The TMEM63 family proteins (A, B, and C), calcium-permeable channels in animals that are preferentially activated by hypo-osmolality, have been implicated in various physiological functions. TMEM63s, together with its plant orthologues OSCAs, are members of a newly identified OSCA/TMEM63 cation channel family that are activated by mechanical forces of osmolality. TMEM63 has three members, TMEM63A, B and C in most animals including mouse and human. TMEM63C is essential for maintaining the kidney filtration barrier integrity in zebrafish, and expresses low in chronic kidney disease patients.

Using single-particle cryo-EM, we determined the structure of TMEM63C at 3.56 Å resolution as a monomer. TMEM63C contains 11 transmembrane helices (TMs), TM0-TM10. The N-terminus is oriented towards the extracellular space, while the C-terminus faces the cytosol. Between TM2 and TM3, there is a long cytosolic domain mainly formed by α-helices. Similar to OSCA, the ion-passing pore of TMEM63C is surrounded by TM3-7. The results show that TMEM63C is in closed state with two restriction sites, the radii of which is smaller than 1 Å. Three bulky pore-facing residues (F542, F543 and Y546 on TM6), highly conserved among TMEM63 and OSCA, have been proposed to play critical roles in channel activities. Particularly, the short α-helix located at the cytoplasmic side of TM6 (TM6b) swung to TM4 to avoid the clash with TM0, the intracellular half of which moved close to TM6, compared to that in OSCA. The movement of TM6b may narrow the ion-passing pore of TMEM63C for calcium entrance. Additionally, we identified two non-protein densities within our cryo-EM map of TMEM63C, which are likely composed of lipids, and may contribute to the modulation of mechanosensitive ion channels gating.

> MSAFPDSMDQKFHNMTVNECFQSRSTVLQGQPFGGIPTVLVLNIILWVFVVLLYSFLRKAAWDYGRLALLIHNDSLTSLIYGEQSEKSSPSEVSLEAERRDRGFSSWFFNSLTMRDRDLINKCGDDARIYITFQYHLIIFVLILCIPSLGIILPVNYIGTVLDWNSHFGRTTIVNVSTESKFLWLHSLFAFLYFLINLAFMGHHCLGFVPKKSLHFTRTLMITYVPTEIQDPEIISKHFHEAYPGCVVTRVHFCYDVRNLIDLDDQRRHAMRGRLYYTAKAKKTGKVMIKTHPCSRLCFCKCWTCFKEVDAEQYYSELEEQLTDEFNAELNRVQLKRLDLIFVTFQDARTVRRIYDDYKYIHCGRHPKQSSVTTIVKNYHWRVAHAPHPKDIIWKHLSIRRFSWWTRFIAINTFLFFLFFFLTTPAIIINTIDIYNVTRPIEKLQSPIVTQFFPSVLLWAFTVTMPLLVYLSAFLEAHWTRSSQNLIIVHKCYIFLVFMVVILPSMGLTSLHVFLRWLFDIYYLEHATIRFQCVFLPDNGAFFINYVITAALLGTGMELMRLGSLCTYCTRLFLSKSEPERVHIRKNQATDFQFGREYAWMLNVFSVVMAYSITCPIIVPFGLLYLCMKHITDRYNMYYSYAPTKLNAQIHMAAVYQAIFAPLLGLFWMLFFSILRVGSLHSITLFSMSSLIISVVIAFSGVFLGKLRIAQRYEQPEEETETVFDVEPSSTTSTPTSLLYVATVLQEPELNLTPASSPARHTYGTINSQPEEGEEESGLRGFARELDSAQFQEGLEMEGQSH>[6x]SSLVRRIISTAKAPAAIGPYSQAVLVDRTIYISGQLGMDPASGQLVPGGVVEEAKQALTNIGEILKAAGCDFTNVVKATVLLADI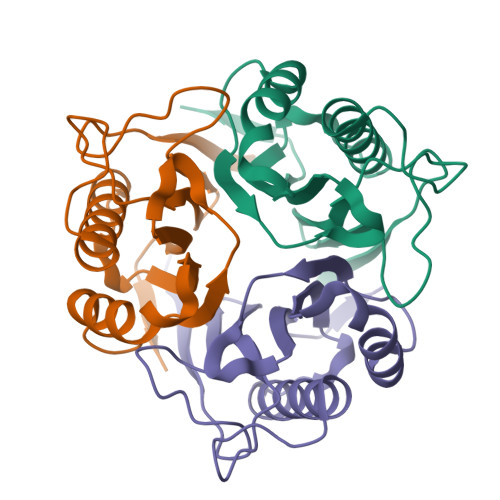NDFSAVNDVYKQYFQSSFPARAAYQVAALPKGGRVEIEAIAVQGPLTTASL>MDHRTSIAQAMVDRISKQMDGSQPDEYFNNLYGNVSRQTYKFEEIREFPYVAVH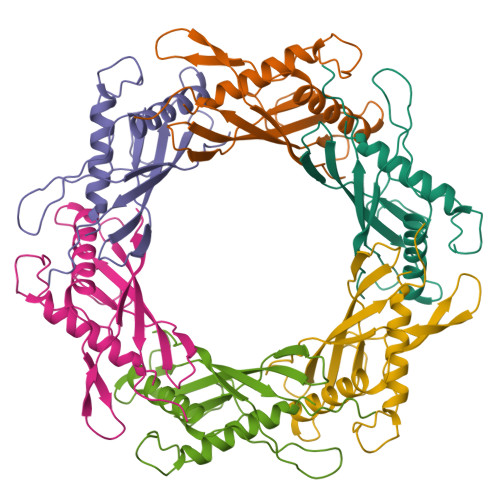IGTETGQYLPSGQQWMFLELPILVYDKEKTDIQEQLEKLVADIKTVIDTGGNLEYTVSKPNGSTFPCEATDMIITSVSTDEGLLAPYGLAEINVTVRYQPPRRSLRR[6x]> GATAEKQKHDGRVKIGHYILGDTLGVGTFGKVKVGKHELTGHKVAVKILNRQKIRSLDVVGKIRREIQNLKLFRHPHIIKLYQVISTPSDIFMVMEYVSGGELFDYICKNGRLDEKESRRLFQQILSGVDYCHRHMVVHRDLKPENVLLDAHMNAKIADFGLSNMMSDGE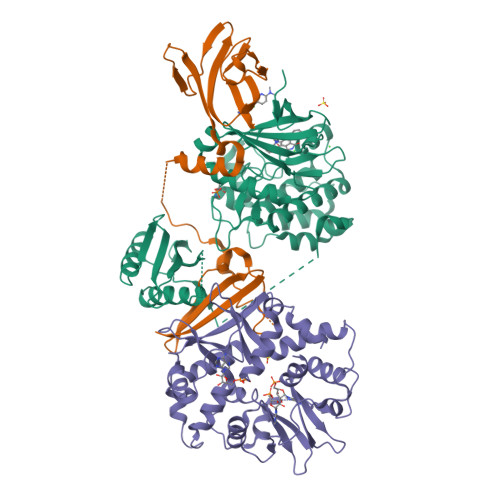FLRTSCGSPNYAAPEVISGRLYAGPEVDIWSSGVILYALLCGTLPFDDDHVPTLFKKICDGIFYTPQYLNPSVISLLKHMLQVDPMKRATIKDIREHEWFKQDLPKYLFPEDPSYSSTMIDDEALKEVCEKFECSEEEVLSCLYNRNHQDPLAVAYHLIIDNRRIMNEAKDFYLATSPPDSFLDDHHLTRPHPERVPFLVAETPRARHTLDELNPQKSKHQGVRKAKWHLGIRSQSRPNDIMAEVCRAIKQLDYEWKVVNPYYLRVRRKNPVTSTFSKMSLQLYQVDSRTYLLDFRSIDDEASGGPGGSAPRPGSHTIEFFEMCANLIKILAQ;> MEVNEKAPAQARPTVFRWTGGGKEVYLSGSFNNWSKLPLTRDHNNFVAILDLPEGEHQYKFFVDGQWTHDPSEPIVTSQLGTVNNIIQVKKTDFEVFDALMVDSQKCSDVSELSSSPPGPYHQEPYISKPEERFKAPPILPPHLLQVILNKDTGISCDPALLPEPNHVMLNHLYALSIKDGVMVLSATHRYKKKYVTTLLYKPI;> MESVAAESAPAPENEHSQETPESNSSVYTTFMKSHRCYDLIPTSSKLVVFDTSLQVKKAFFALVTNGVRAAPLWDSKKQSFVGMLTITDFINILHRYYKSALVQIYELEEHKIETWREVYLQDSFKPLVCISPNASLFDAVSSLIRNKIHRLPVIDPESGNTLYILTHKRILKFLKLFITEFPKPEFMSKSLEELQIGTYANIAMVRTTTPVYVALGIFVQHRVSALPVVDEKGRVVDIYSKFDVINLAAEKTYNNLDVSVTKALQHRSHYFEGVLKCYLHETLEAIINRLVEAEVHRLVVVDEHDVVKGIVSLSDILQALVLTGGEKKP> MTTAIVPRVSGGEEEHGHLEEFRTDPIGLMQRVRDECGDVGWFQLANKHVVLLSGAKANEFFFRSSDEELDQAE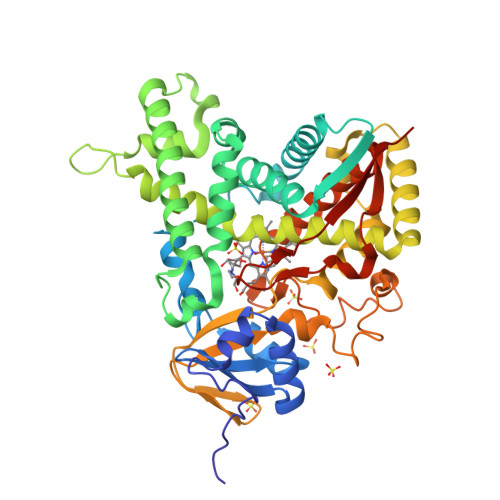AYPFMTPIFGKGVVFDASPERRKEMLHNSALRGEHMKGHATTIEREVHRMIENWGQEGEIDLLEFFAELTIYTSTSCLIGTKFRNQLDSRFAHFYHELERGTDPLCYVDPYLPIESFRRRDEARKGLVALVQDIMHQRVANPPTDKRDRDMLDVLVSITDEQGNPRFCADEVTGMFISLMFAGHHTSSGTSAWTLIELLRHPDAYAAVIDELDELYADGQPVSFHALRQIPRLENVLKETLRLHPPLIILMRVAKGEFQVEGYPIHEGELVAASPAISNRIAEDFPDPDEFVPERYQEPRQEDLINRWTWIPFGAGRHRCVGAAFATMQIKAIFSVLLREYEFEMAQPADSYRNDHSKMVVQLARPARVRYRRRKMSDNRGH> SNAMASGGSGGVSVPALWSEVNRYGQNGDFTRALKTVNKILQINKDDVTALHCKVVCLIQNGSFKEALNVINTHTKVLANNSLSFEKAYCEYRLNRIENALKTIESANQQTDKLKELYGQVLYRLERYDECLAVYRDLVRNSQDDYDEERKTNLSAVVAAQSNWEKVVPENLGLQEGTHELCYNTACALIGQGQLNQAMKILQKAEDLCRRSLSEDTDGTEEDPQAELAIIHGQMAYILQLQGRTEEALQLYNQIIKLKPTDVGLLAVIANNIITINKDQNVFDSKKKVKLTNAEGVEFKLSKKQLQAIEFNKALLAMYTNQAEQCRKISASLQSQSPEHLLPVLIQAAQLCREKQHTKAIELLQEFSDQHPENAAEIKLTMAQLKISQ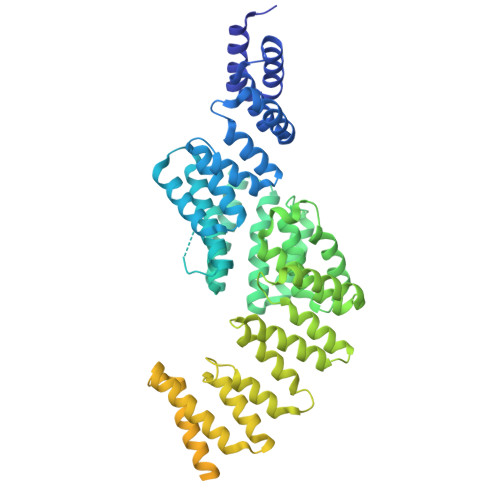GNISKACLILRSIEELKHKPGMVSALVTMYSHEEDIDSAIEVFTQAIQWYQNHQPKSPAHLSLIREAANFKLKYGRKKEAISDLQQLWKQNPKDIHTLAQLISAYSLVDPEKAKALSKHLPSSDSMSLKVDVEALENSAGATYIRKKGGKVTGDSQPKEQGQGDLKKKKKKKKGKLPKNYDPKVTPDPERWLPMRERSYYRGRKKGKKKDQIGKGTQGATAGASSELDASKTVSSPPTSPRPGSAATVSASTSNIIPPRHQKPAGAPATKKKQQQKKKKGGKGGW> GGCUUAUCAAGAGAGGGUGAGCGACUGGCGCGAAGAGCCCCGGCAACCAGAAAUGGUGCC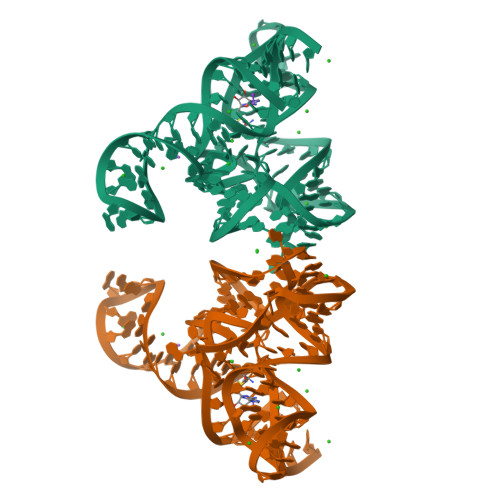AAUUCCUGCAGCGGAAACGUUGAAAGAUGAGCCG>[3x]MKMNRRNVLVGLGTIVAGGGAALGTGAFSSVEADRTVSVAVAGDASSALAFDTSDSNGNQYSDASSITNGTLELAFDS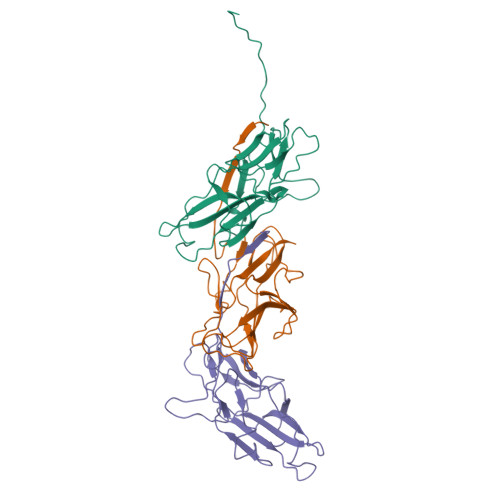LGNSSGINLGAKTTFSPLFRTINNGSNNVNLSIYSSEGTIQTSPTILDSYNAVIENTINDGNGNSLTIEYAFTDENDNSIVGDGTNGSSVSLDATGGSDPNEEVSLVIGVADPGSSFDPSTTISGYLSEVTIVASSV(3P,5M)-3-[3-(1-cyclobutylpiperidin-4-yl)phenyl]-5-(1H-tetrazol-5-yl)-2,1-benzoxazole | C23 H24 N6 O | 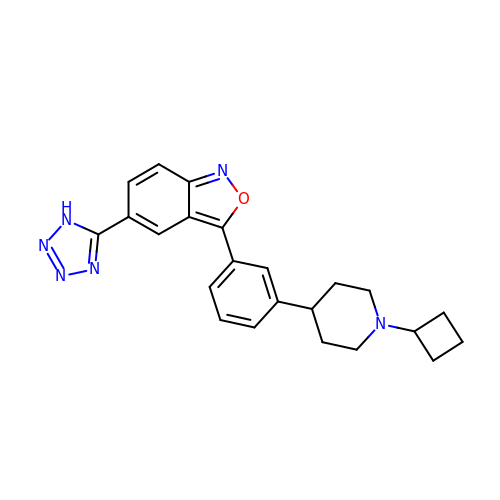JZWSGCNSEOEUCD-UHFFFAOYSA-N>[7x]MADSDINIKTGTTDIGSNTTVKTGDLVTYDKENGMHKKVFYSFIDDKNHNKKLLVIRTKGTIAGQYRVYSEEGANKSGLAWPSAFKVQLQLPDNEVAQISDYYPRNSIDTKEYMSTLTYGFNGNVTGDDTGKIGGLIGANVSIGHTLKYVQPDFKTILESPTDKKVGWKVIFNNMVNQNAGPYDRDSWNPVYGNQLFMKTANGSMKAAENFLDPNKASSLLSSGFSPDFATVITMDRKASKQ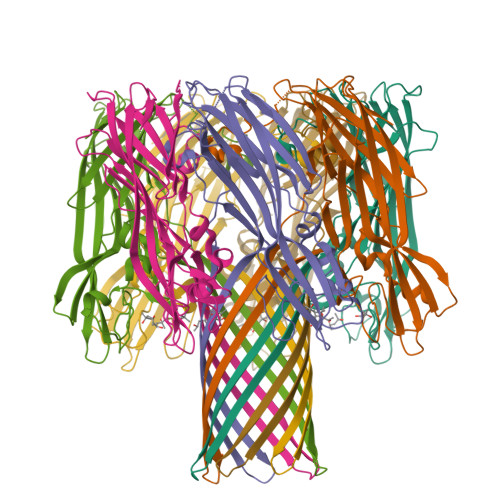QTNIDVIYERVRDDYQLHWTSTNWKGTNTKDKWTDRSSERYKIDWEKEEMTNLEHHHHHH2-cyanoacetamide | C3 H4 N2 O | 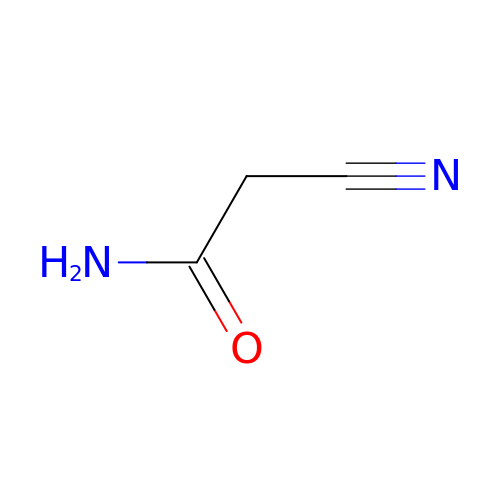DGJMPUGMZIKDRO-UHFFFAOYSA-N>[12x]MKYDTSELCDIYQEDVNVVEPLFSNFGGRASFGGQIITVKCFEDNGLLYDLLEQNGRGRVLVVDGGGSVRRALVDAELARLAVQNEWEGLVIYGAVRQVDDLEE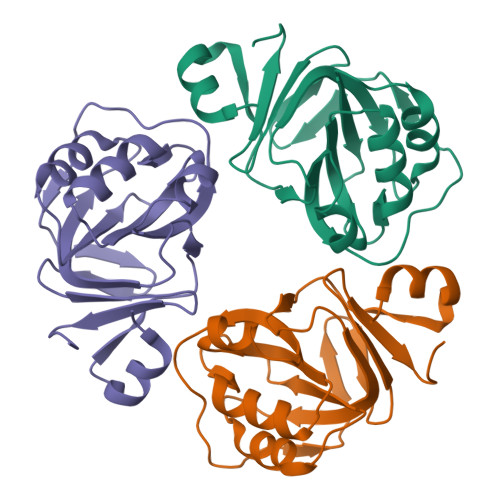LDIGIQAMAAIPVGAAGEGIGESDVRVNFGGVTFFSGDHLYADNTGIILSEDPLDIE> FNKECLLRYKEAALDPNLNLYQRIAKIVSI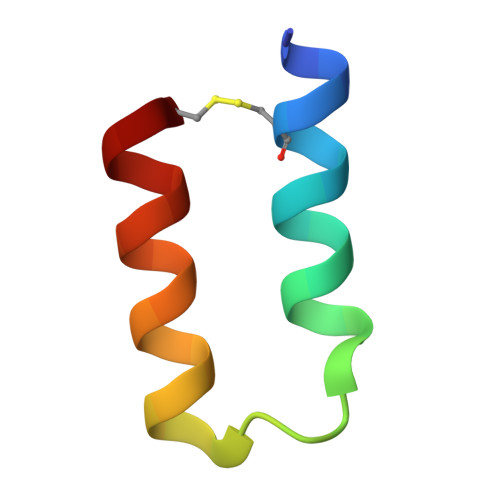DDDC> GPGSMTDFPKLNRIKSDDENMEKIHVAARKGQTDEVRRLIETGVSPTIQNRFGCTALHLACKFGCVDTAKYLASVGEVHSLWHGQKPIHLAVMANKTDLVVALVEGAKERGQMPESLLNECDEREVNEIGSHVKHCKGQTALHWCVGLGPEYLEMIKILVQLGASPTAKDKADETPLMRAMEFRNREALDLMMDTVPSKSSLRLDYANKQGNSHLHWAILINWEDVA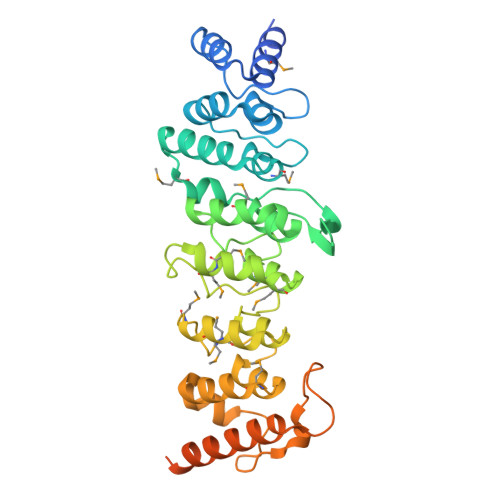MRFVEMGIDVNMEDNEHTVPLYLSVRAAMVLLTKELLQKTDVFLIQACPYHNGTTVLPDRVVWLDFVPAAADPSKQEVLQLLQEKLDEVVRSLNTGAGGAVKRKKKAAPAVKRMKLAPSAPVRTRSRSRARSSAVSK> TTPLVHVASVEKGRSYEDFQKVYNAIALKLREDDEYDNYIGYGPVLVRLAWHTSGTWDKHDNTGGSYGGTYRFKKEFNDPSNAGLQNGFKFLEPIHKEFPWISSGDLFSLGGVTAVQEMQGPKIPWRCGRVDTPEDTTPDNGRLPDADKDADYVRTFFQRLNMNDREVVALMGAHAL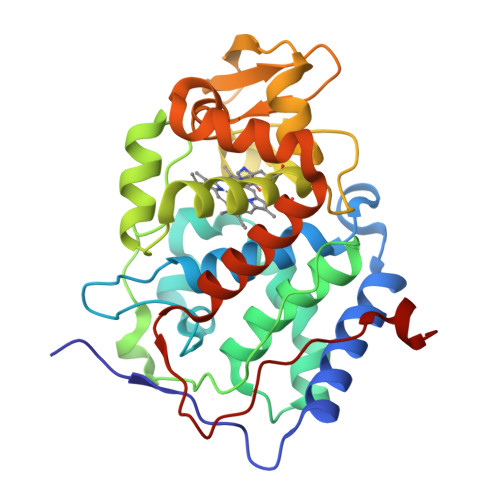GKTHLKNSGYEGPWGAANNVFTNEFYLNLLNEDWKLEKNDANNEQWDSKSGYMMLPTDYSLIQDPKYLSIVKEYANDQDKFFKDFSKAFEKLLEDGITFPKDAPSPFIFKTLEEQGL6-[(2R)-2-(3-fluorophenyl)pyrrolidin-1-yl]-3-(pyridin-2-yl)imidazo[1,2-b]pyridazine 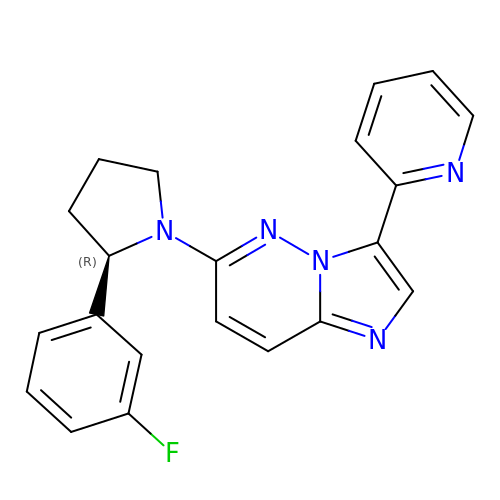| C21 H18 F N5 | RKERQEKFTWWCEY-GOSISDBHSA-N>[2x]GMDMKKHGLSIGINRIESVFFVTLKAIGTLTHEDYLVITPMLEGALSQVDQPKVSLFLDATELDGWDLRAAWDDLKLGLKHK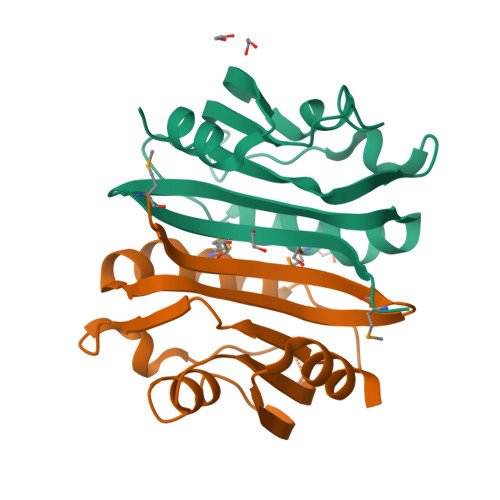SEFERVAILGNKDWQEWAAKIGSWFIAGEIKYFEDEDDALKWLRY> GLIVDTRDVEERVHVMRETKLAPTVAHGVFNPEFGPAALSNKDPRLNEGVVLDEVIFSKHKGDTKMSAEDKALFRRCAADYASRLHSVLGTANAPLSIYEAIKGVDGLDAMEPDTAPGLPWALQGKRRGALIDFENGTVGPEVEAALKLMEKREYKFACQTFLKD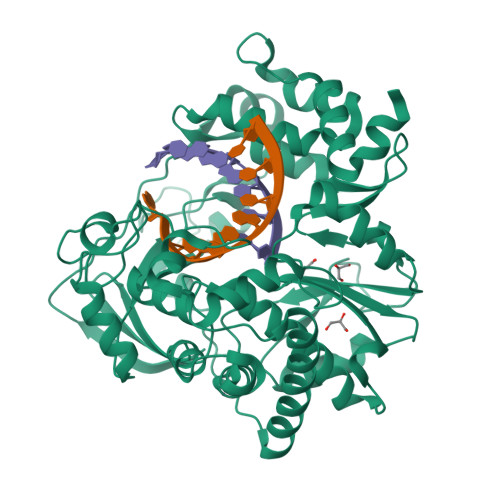EIRPMEKVRAGKTRIVDVLPVEHILYTRMMIGRFCAQMHSNNGPQIGSAVGCNPDVDWQRFGTHFAQYRNVWDVDYSAFDANHCSDAMNIMFEEVFRTEFGFHPNAEWILKTLVNTEHAYENKRITVEGGMPSGCSATSIINTILNNIYVLYALRRHYEGVELDTYTMISYGDDIVVASDYDLDFEALKPHFKSLGQTITPADKSDKGFVLGHSITDVTFLKRHFHMDYGTGFYKPVMASKTLEAILSFARRGTIQEKLISVAGLAVHSGPDEYRRLFEPFQGLFEIPSYRSLYLRWVNAVCGDAAAALEHHHHHH>[2x]CCTCTGGTCTCC;>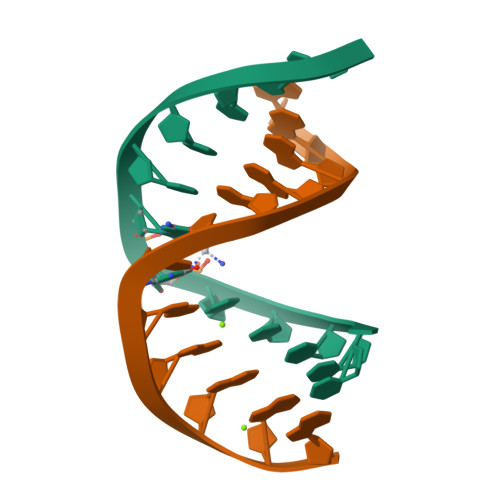[2x]GGAGACCAGAGG>GMVGSLNCIVAVSQNMGIGKNGDLPWPPLRNEFRYFQRMTTTSSVEGKQNLVIMGKKTWFSIPEKNRPLKGRINLVLSRELKEPPQGAHFLSRSLDDALKLTEQPELANKVDMVWIVGGSSVYKEAMNHPGHLKLFVTRIMQDFESDTFFPEIDLE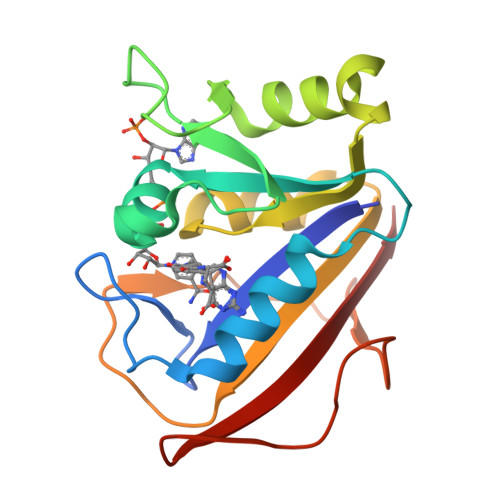KYKLLPEYPGVLSDVQEEKGIKYKFEVYEKND[4x]> SNAGKALVIVESPAKAKTINKYLGSDYVVKSSVGHIRDLPTSGSAAKKSADSTSTKTAKKPKKDERGALVNRMGVDPWHNWEAHYEVLPGKEKVVSELKQLAEKADHIYLATDLDREGEAIAWHLREVIGGDDARYSRVVFNEITKNAIRQAFNKPGELNIDRVNAQQARRFMDRVVGYMVSPLLWKKIARGLSAGRVQSVAVRLVVEREREIKAFVPEEFWEVDASTTTPSGEALALQVTHQNDKPFRPVNKEQTQAAVSLLEKARYSVLEREDKPTTSKPGAPFITSTLQQAASTRLGFGVKKTMMMAQRLYEAGYITYMRTDSTNLSQDAVNMVRGYISDNFGKKYLPESPNQYASKENSQEAHEAIRPSDVNVMAESLKDMEADAQKLYQLIWRQFVACQMTPAKYDSTTLTVGAGDFRLKARGRILRFDGWTKVMPALRKGDEDRILPAVNKGDALTLVELTPAQHFTKPPARFSEASLVKELEKRGIGRPSTYASIISTIQDRGYVRVENRRFYAEKMGEIVTDRLEENFRELMNYDFTAQMENSLDQVANHEAEWKAVLDHFFSDFTQQLDKAEKDPEEGGMRPNQMVLTSIDCPTCGRKMGIRTASTGVFLGCSGYALPPKERCKTTINLVPENEVLNVLEGEDAETNALRAKRRCPKCGTAMDSYLIDPKRKLHVCGNNPTCDGYEIEEGEFRIKGYDGPIVECEKCGSEMHLKMGRFGKYMACTNEECKNTRKILRNGEVAPPKEDPVPLPELPCEKSDAYFVLRDGAAGVFLAANTFPKSRETRAPLVEELYRFRDRLPEKLRYLADAPQQDPEGNKTMVRFSRKTKQQYVSSEKDGKATGWSAFYVDGKWVEGKK

Escherichia coli topoisomerase I (EcTOP1) encoded by the topA gene is the prototype type IA topoisomerase required for preventing excess negative DNA supercoiling. It has an important role in removing transcription-induced negative supercoiling behind the RNA polymerase complex. Type IA topoisomerases act on a single-stranded region of DNA to initiate change in DNA topology by creating a break on the G-strand of DNA. The C-terminal domains of EcTOP1 are essential for the enzyme to have the capability of removing negative supercoils from DNA rapidly in a processive mechanism.

Here, we present for the first time the structure of completely active full-length EcTOP1 in complex with single-stranded DNA (ssDNA). There is one full-length EcTOP1 molecule in the asymmetric unit. As revealed in this study, TOP30C actually contains three 4-Cys zinc ribbon domains (D5–D7) and two zinc ribbon-like domains (D8–D9). In the structure of full-length EcTOP1 in complex with DNA, the ssDNA segment is bound to TOP30C with its 3′-OH end primarily interacting with D5. The extended ssDNA also interacts with D7, D8 and D9 but not D6. Each domain comprises a 4-stranded antiparallel β-sheet with a Zn(II)-binding site on the top of the domain. The Zn(II) ion is coordinated by four conserved cysteines from the β1-β2 and β3-β4 loops. Binding primarily involves parallel π-stacking interactions between the guanine ring moieties of G29 and G28 to the aromatic side chains of the residues Y622 and F616, respectively. Residue R189 is the only residue from TOP67 that contributes to ssDNA binding with two salt-bridges to the backbone phosphate groups of G29 and G28 and a hydrogen bond to the phosphate group of G29. However, it is D6 that forms extensive interactions with TOP67, mostly through its unique helix (α1 of D6).>MATHHTLWMGLALLGVLGDLQAAPEAQVSVQPNFQQDKFLGRWFSAGLASNSSFLREKKAALSMAKSVVAPATDGGLNLTSTFLRKNQCETRTMLLQPAGSLGSYSYRSPHFGSTYSVSVVETDYDQYALLYSQGSKGPGEDFRMATLYSRTQTPRAELKEKFTAFCKAQ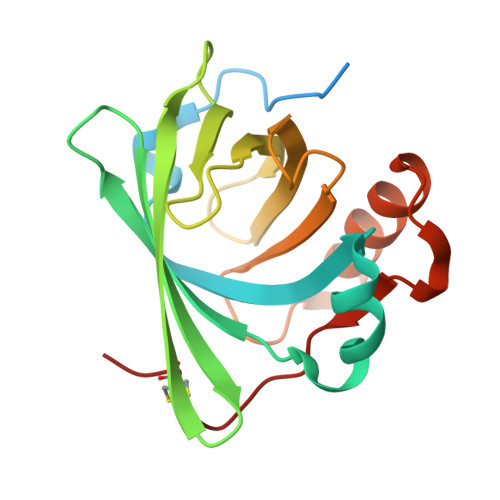GFTEDTIVFLPQTDKCMTEQ[2x]> IVGGQECKD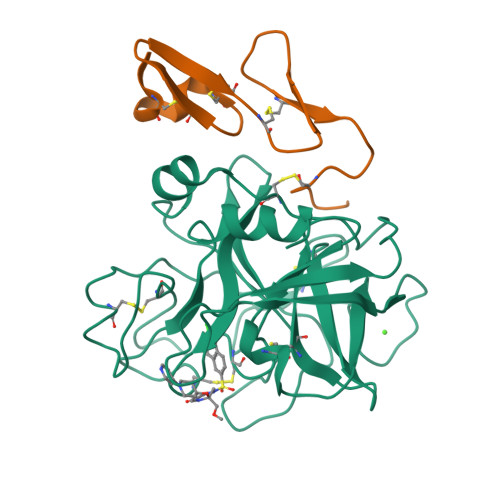GECPWQALLINEENEGFCGGTILSEFYILTAAHCLYQAKRFKVRVGDRNTEQEEGGEAVHEVEVVIKHNRFTKETYDFDIAVLRLKTPITFRMNVAPACLPERDWAESTLMTQKTGIVSGFGRTHEKGRQSTRLKMLEVPYVDRNSCKLSSSFIITQNMFCAGYDTKQEDACQGDSGGPHVTRFKDTYFVTGIVSWGEGCARKGKYGIYTKVTAFLKWIDRSMKTR;> YKDGDQCETSPCQNQGKCKDGLGEYTCTCLEGFEGKNCELFTRKLCSLDNGDCDQFCHEEQNSVVCSCARGYTLADNGKACIPTGPYPCGKQTLER>GAMVNCGHVTAYGPGLTHGVVNKPATFTVNTKDAGEGGLSLAIEGPS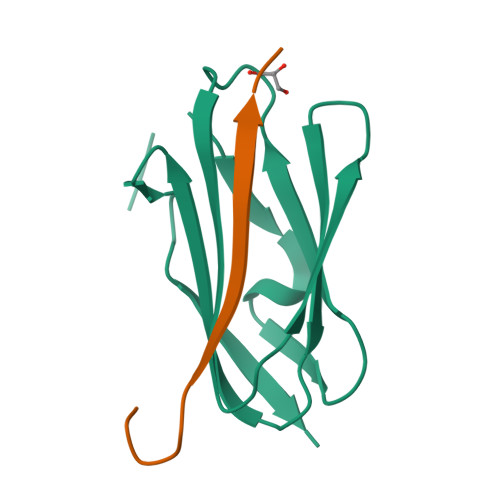KAEISCTDNQDGTCSVSYLPVLPGDYSILVKYNEQHVPGSPFTARVTGDD[2x];>[2x]LRGSLPTFRSSLFLWVRPNGRV N,N-dicyclohexyl-3-(2,4-dichlorophenyl)-5-methyl-1,2-oxazole-4-carboxamide 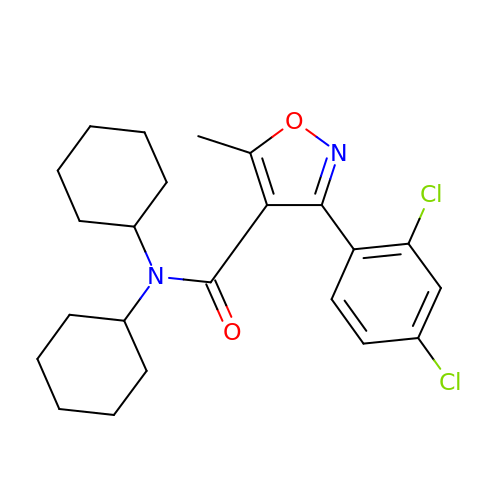| C23 H28 Cl2 N2 O2 | SFPRPAWSWIQRDL-UHFFFAOYSA-N>PLRMGGNGQLQYWPFSSSDLYNWKNNNPSFSEDPGKLTALIESVLTTHQPTWDDCQQLLGTLLTGEEKQRVLLEARKAVRGNDGRPTQLPNEVDAAFPLERPDWDYTTQRGRNHLVLYRQLLLAGMQNAGRSPTNLAKVKGITQGPNESPSAFLERLKEAYRRYTPYDPEDPGQETNVSMSFIWQSAPDIGRKLERLEDLKSKTLGDLVREAEKIFNKRETPEEREERIRRETEEK[4x]

Immature retroviruses are built by the Gag polyprotein; Gag is then cut into domains, and the resulting CA capsid proteins form the mature capsid, which can mediate infection of a new cell. Murine leukemia virus (MLV), the prototypic member of the γ-retroviruses, is commonly used in comparative studies and as a basis for retroviral vector design. The CA domain and immediate downstream residues mediate protein interactions in the immature shell, and, following proteolytic cleavage, CA forms the mature viral capsid. In this study, we have determined the structure of the truncated MLV CA-CTD by X-ray crystallography and have resolved the architecture and CA lattice structures of immature and mature MLV particles by cryo-ET and subtomogram averaging.

We identified 1,299 pentamerically coordinated positions from the 134 virions in our dataset, extracted subtomograms at these positions, and iteratively aligned and averaged them to generate a structure of the mature MLV CA pentamer at a resolution of 8.6 Å. CA domains were fitted into the map as rigid bodies. The CA-CTD layer displays high curvature at the pentamer positions, and the CA-NTD pentamer protrudes further outward from the CA-CTD layer than in the hexamer. Comparison of the interfaces between neighboring CA molecules in the pentamer and hexamer revealed subtle differences in these interactions but no dramatic opening of the interdomain cleft as we previously observed in the HIV-1 pentamer. The MLV CA-NTD pentamer is more tightly packed around the fivefold symmetry axis than the hexamer, resulting in an even narrower pore in the center and higher local positively charged electric potential contributed by arginines in the β-hairpin. The mature MLV cores consisted of flat areas of lattice joined at seams with locally higher curvature, and with pentamers positioned at the highly curved vertices. Within spiral or nested cores, more than 12 pentamers are required to accommodate the increased total curvature, and we observed as many as 24 pentamers within a single virus particle (Fig. 4B1). As the total curvature of a multilayered structure is greater than that in a sphere, more than 12 pentamers are present in MLV particles. The presence of pentamers, rather than gaps as in the immature lattice, suggests that having a CA lattice without holes may be important during early stages of the MLV lifecycle.> MAATVPS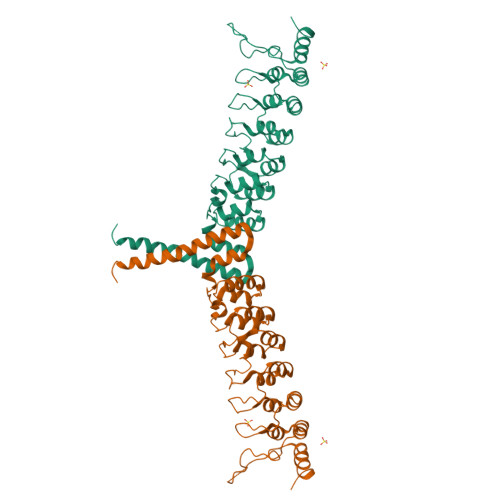RDSGEEAAEPSAPSRTPQCEPQAPEMLQRAREYNARLFGLAQRSARALLDYGVTADARALLAGQRHLLTAQDENGDTPLHLAIIHGQTSVIEQIVYVIHHAQDLGVVNLTNHLHQTPLHLAVITGQTSVVSFLLRVGADPALLDRHGDSAMHLALRAGAGAPELLRALLQSGAPAVPQLLHMPDFEGLYPVHLAVRARSPECLDLLVDSGAEVEATERQGGRTALHLATEMEELGLVTHLVTKLRANVNARTFAGNTPLHLAAGLGYPTLTRLLLKAGADIHAENEEPLCPLPSPPTSDSDSDSEGPEKDTRSSFRGHTPLDLTCSTKVKTLLLNAAQNTMEPPLTPPSPAG>[2x]TADSRKTYTLTDYLKNTYRLKLYSLRWISDHEYLYKQENNILVFNAEYGNSSVFLENSTFDEFGHSINDYSISPDGQFILLEYNYVKQWRHSYTASYDIYDLNKRQLITEERIPNNTQWVTWSPVGHKLAYVWNNDIYVKIEPNLPSYRITWTGKEDIIYNGITDWVYEEEVFSAYSALWWSPNGTFLAYAQFNDTEVPLIEYSFYSDESLQYPKTVRVPYPKAGAVNPTVKFFVVNTDSLSSVTNATSIQITAPASM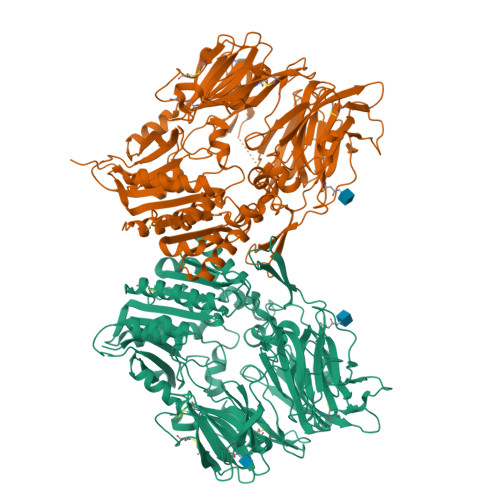LIGDHYLCDVTWATQERISLQWLRRIQNYSVMDICDYDESSGRWNCLVARQHIEMSTTGWVGRFRPSEPHFTLDGNSFYKIISNEEGYRHICYFQIDKKDCTFITKGTWEVIGIEALTSDYLYYISNEYKGMPGGRNLYKIQLSDYTKVTCLSCELNPERCQYYSVSFSKEAKYYQLRCSGPGLPLYTLHSSVNDKGLRVLEDNSALDKMLQNVQMPSKKLDFIILNETKFWYQMILPPHFDKSKKYPLLLDVYAGPCSQKADTVFRLNWATYLASTENIIVASFDGRGSGYQGDKIMHAINRRLGTFEVEDQIEAARQFSKMGFVDNKRIAIWGWSYGGYVTSMVLGSGSGVFKCGIAVAPVSRWEYYDSVYTERYMGLPTPEDNLDHYRNSTVMSRAENFKQVEYLLIHGTADDNVHFQQSAQISKALVDVGVDFQAMWYTDEDHGIASSTAHQHIYTHMSHFIKQCFSLP>[3x]GPTNFEKEYDLEKLVNNSLDLLSIQRLDGTVLQVNPAFERLLGWREEELIGRNPFHLLHPEDRESTFQEFKKLNQGLPVFAFQNRFLCSDGTYKYFSWTASPDLSAGLIYVTGRDI

The long-wavelength beamline I23 at Diamond Light Source overcomes these limitations and extends the accessible wavelength range to λ = 5.9 Å. In this study, we report the determination of diverse protein structures by experimental phasing techniques carried out at long wavelengths on beamline I23 at Diamond Light Source using S, Ca, K, Cl, V, I, Cd, and P as anomalous scatterers. Native-SAD uses light atoms naturally occurring in proteins or bound to proteins. We demonstrate that long-wavelength native-SAD has become a very compelling technique, where a low multiplicity dataset from a single crystal can be sufficient for successful structure determination, making it a general vehicle of choice for experimental phasing.

Amongst the structures solved at the beamline, the lowest sulfur content was found in the PAS domain of the protein codified by the locus tag LIC_11128 from Leptospira interrogans serovar Copenhageni Fiocruz L1-130. The domain contains only one sulfur in 116 amino acids (0.9% sulfur content), nevertheless the substructure solution was straightforward in SHELXD22 with 360° of data, a resolution of 2.5 Å, completeness of 83% and an overall multiplicity of 11. For refinement purposes, additional datasets were included, resulting in a final multiplicity of 49.2.>[4x]MKNFEIVTVTPDHAEQLISMIHELAEFEKMKSSVVNTAEKLRKDIENKAVHGFIAFIGEEP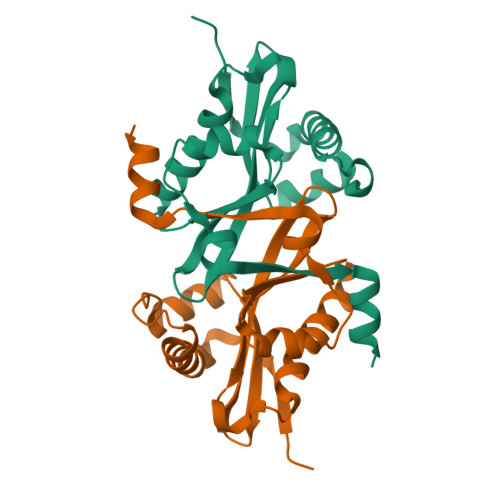AGMNLFYYAYSTWVGQYLHMEDLYIRPQFRRMGLARTLWKKLAELARDKGIVRLEWAVLDWNKNAIALYDTVDYVNLTKSEGWFTFRMDGAAINKFADE> MTDESKPTDDQPTSKG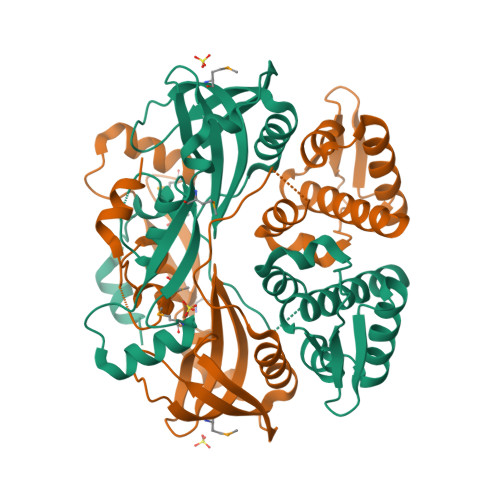RQGARWGQERRLEFIDYRLRWDGQINRSSLTDFFGISVPQASLDITEYAKLAESNLEYDTRARVYRATESFKAVFPSSAVERYLDDLLRVAVQPEIPYGSFLGWQSPVAAVPKLGRRLNADIVGVILRAIRETGFIEVFYQSLTDPEGGERMLSPHALVHDGNRWHVRAYCHKRKAFRDFSLTRIKCCKYVGQDRDRADEDYAWNTMVNVVLTPHPGLTPAQRKLIENDFLMEGGEMHVECRRALLLYLLFQLNLNEDQADQRPEVIQLALKNRDEIKDLIQY The membrane protein Dispatched (Disp), which belongs to the RND family of small molecule transporters, is essential for Hedgehog (Hh) signaling, by catalyzing the extracellular release of palmitate- and cholesterol-modified Hh ligands from producing cells. Also uniquely among RND proteins, Disp activity requires Furin-mediated cleavage at a conserved site in its first large extracellular domain (ECD1), yielding a mature Disp protein consisting of two non-covalently associated fragments.

Importantly, upon incubation with 3C protease, hDisp1NNN-3C was quantitatively cleaved into a larger band and two smaller bands, similar to purified hDisp1NNN; this indicates that our hDisp1NNN-3C construct is suitable for generating pure hDisp1 in either cleaved and uncleaved state. We solved the structure of uncleaved hDisp1NNN-3C at overall resolution of 3.61 Å, and the structure of hDisp1NNN-3C-cleaved at 3.68 Å. A comparison between the structures of hDisp1NNN-3C and hDisp1NNN-3C-cleaved reveals conformational shifts of the two ECDs, whereas the TMDs remain largely unchanged. After proteolytic cleavage, the two ECDs turn outwardly, away from each other, by approximately 2–3 Å, leading to a more open conformation of the extracellular surface of hDisp1. Additionally, density peaks for the C-loop in ECD1 were observed in the map of hDisp1NNN-3C-cleaved, enabling us to build 6 residues (residues 279–284) in the C-loop. The resolved C-loop is moved away from ECD2 in hDisp1NNN-3C-cleaved, suggesting that the uncleaved C-loop perhaps restricts the motions of the two ECDs, and that proteolytic cleavage allows them to move away from each other. Four N-linked glycosylation sites were identified in both hDisp1 structures, Asn363 and Asn476 on ECD1, and Asn836 and Asn917 on ECD2, which, in turn, validated sequence assignment. Similar to the sterol-like molecules seen in the reported Ptch1 cryo-EM structures, we observed several sterol-like molecules in the transmembrane domain (TMD) of both our hDisp1 structures; we assigned these molecules to the sterol detergent, cholesteryl hemisuccinate (CHS), which was used for protein purification. In contrast to other RND proteins, such as Ptch123,25,26, in which the ECDs are close together, the two ECDs in hDisp1NNN-3C and hDisp1NNN-3C-cleaved are splayed apart, exhibiting an open conformation, as previously reported for dDisp and hDisp132,33.

> MAMSNGNNDFVVLSNSSIATSAANPSPLTPCDGDHAAQQLTPKEATRTKVSPNGCLQLNGTVKSSFLPLDNQRMPQMLPQCCHPCPYHHPLTSHSSHQECHPEAGPAAPSALASCCMQPHSEYSASLCPNHSPVYQTTCCLQPSPSFCLHHPWPDHFQHQPVQQHIANIRPSRPFKLPKSYAALIADWPVVVLGMCTMFIVVCALVGVLVPELPDFSDPLLGFEPRGTAIGQRLVTWNNMVKNTGYKATLANYPFKYADEQASSLEVLFQ;> GPGSEVDWNFHKDSFFCDVPSDRYSRVVFTSSGGETLWNLPAIKSMCNVDNSRIRSHPQFGDLCQRTTAASCCPSWTLGNYIAILNNRSSCQKIVERDVSHTLKLLRTCAKHYQNGTLGPDCWDMAARRKDQLKCTNVPRKCTKYNAVYQILHYLVDKDFMTPKTADYATPALKYSMLFSPTEKGESMMNIYLDNFENWNSSDGVTTITGIEFGIKHSLFQDYLLMDTVYPAIAIVIVLLVMCVYTKSMFITLMTMFAIISSLIVSYFLYRVVFHFEFFPFMNLTALIILVGIGANNAFVLCDVWNYTKFDKPHAETSETVSITLQHAALSMFVTSFTTAAAFYANYVSNITAIRCFGVYAGTAILVNYVLMVTWLPAVVVLHERYLLNIFTCFKKPQQQIYDNKSCWTVACQKCHKVLFAISEASRIFFEKVLPCIVIKFRYLWLFWFLALTVGGAYIVCINPKMKLPSLELSEFQVFRSSHPFERYDAEYKKLFMFERVHHGEELHMPITVIWGVSPEDNGNPLNPKSKGKLTLDSSFNIASPASQAWILHFCQKLRNQTFFYQTDEQDFTSCFIETFKQWMENQDCDEPALYPCCSHWSFPYKQEIFELCIKRAIMELERSTGYHLDSKTPGPRFDINDTIRAVVLEFQSTYLFTLAYEKMHQFYKEVDSWISSELSSAPEGLSNGWFVSNLEFYDLQDSLSDGTLIAMGLSVAVAFSVMLLTTWNIIISLYAIISIAGTIFVTVGSLVLLGWELNVLESVTISVAVGLSVNFAVHYGVAYRLAPDPDREGKVIFSLSRVGSAMAMAALTTFVAGAMMMPSTVLAYTQLGTFMMLIMCISWAFATFFFQCMCRCLGPQGTCGQIPLPKKLQCSAFSHALSTSPSDKGQSKTHTINAYHLDPRGPKSELEHEFYELEPLASHSCTAPEKTTYEETHICSEFFNSQAKNLGMPVHAAYNSELSKSTESDAGSALLQPPLEQHTVCHFFSLNQRCSCPDAYKHLNYGPHSCQQMGDCLCHQCSPTTSSFVQIQNGVAPLKATHQAVEGFVHPITHIHHCPCLQGRVKPAGMQNSLPRNFFLHPVQHIQAQEKIGKTNVHSLQRSIEEHLPKMAEPSSFVCRSTGSLLKTCCDPENKQRELCKNRDVSNLESSGGTENKAGGKVELSLSQTDASVNSEHFNQNEPKVLFNHLMGEAGCRSCPNNSQSCGRIVRVKCNSVDCQMPNMEANVPAVLTHSELSGESLLIKTL~{N}-[3-[(4~{S})-2-azanyl-4-methyl-5,6-dihydro-1,3-thiazin-4-yl]phenyl]-5-bromanyl-pyridine-2-carboxamide 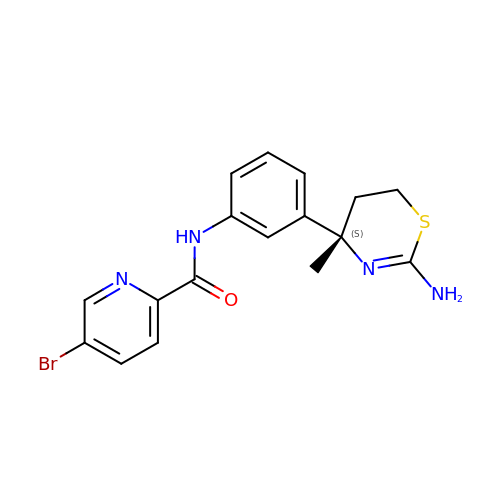| C17 H17 Br N4 O S | FSIYTVBWWROBPT-KRWDZBQOSA-N>GPGSQWNQLQQLDTRYLEQLHQLYSDSFPMELRQFLAPWIESQDWAYAASKESHATLVFHNLLGEIDQQYSRFLQESNVLYQHNLRRIKQFLQSRYLEKPMEIARIVARCLWEESRLLQTAATAAQQGG[5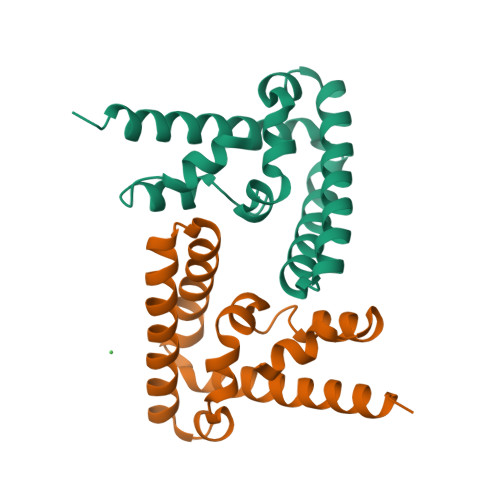x]>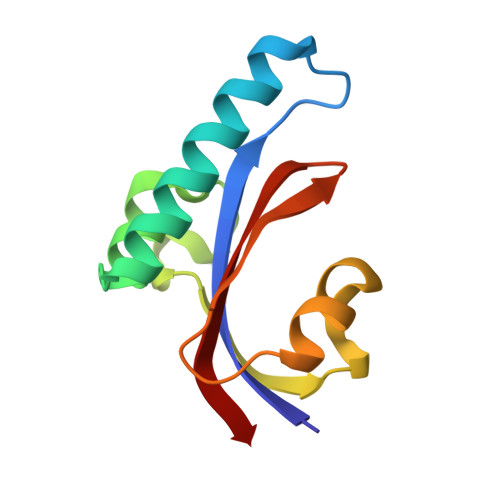 TELNLSHILIPLPENPTSDQVNEAESQARAIVDQARNGADFGKLAIAHSADQQALNGGQMGWGRIQELPGIFAQALSTAKKGDIVGPIRSGVGFHILKVNDLR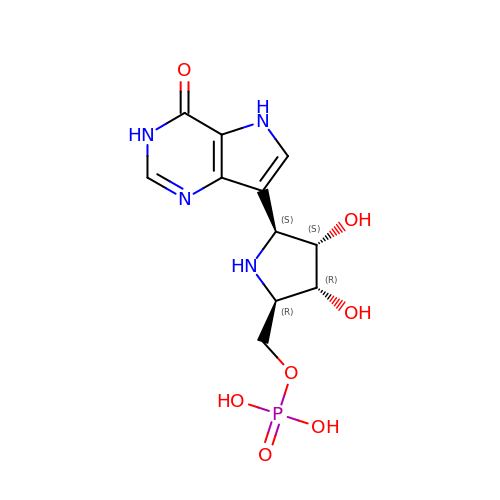(1S)-1(9-DEAZAHYPOXANTHIN-9YL)1,4-DIDEOXY-1,4-IMINO-D-RIBITOL-5-PHOSPHATE | C11 H15 N4 O7 P | VJTAXXUIRYOXBT-KUBHLMPHSA-N> MPVFHTRTIESILEPVAQQISHLVIMHEEGEVDGKAIPDLTAPVAAVQAAVSNLVRVGKETVQTTEDQILKRDMPPAFIKVENACTKLVQAAQMLQSDPYSVPARDYLIDGSRGILSGTSDLLLTFDEAEVRKIIRVCKGILEYLTVAEVVETMEDLVTYTKNLGPGMTKMAKMIDERQQELTHQEHRVMLVNSMNTVKELLPVLISAMKIFVTTKNSKNQGIEEALKNRNFTVE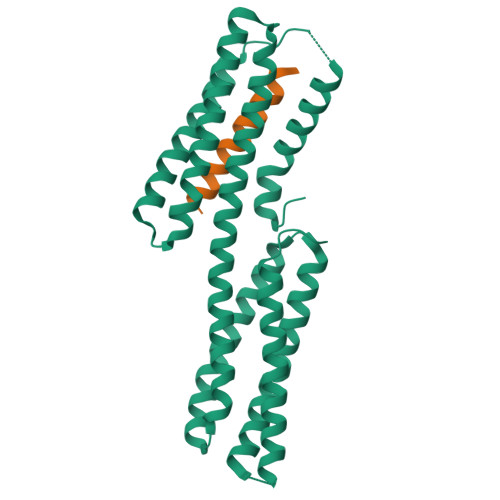KMSAEINEIIRVLQLTSWDEDAW;> ETQVVLINAVKDVAKALGDLISATKAAAG> GPLGSIKELKMSKDEIKREYKEMEGSPE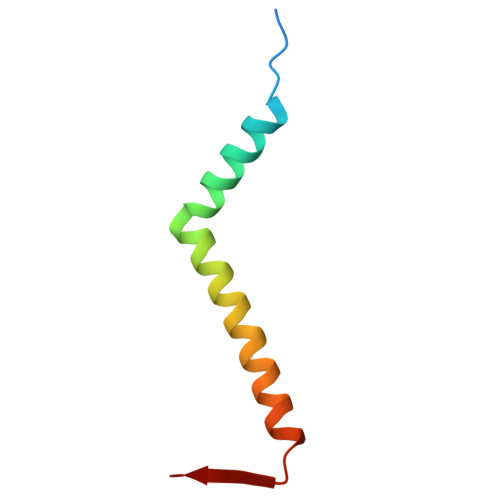IKSKRRQFHQEIQSRNMRENVKRSSVVVAN1,4-DIDEOXY-1,4-IMINO-D-ARABINITOL 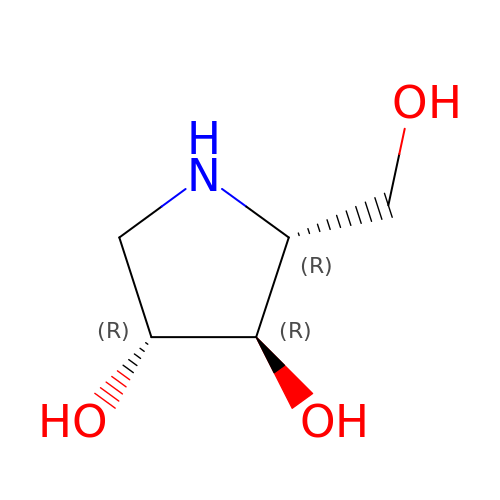| C5 H11 N O3 | OQEBIHBLFRADNM-UOWFLXDJSA-N> MGSSHHHHHSSGLVPRGSHMTTSAAS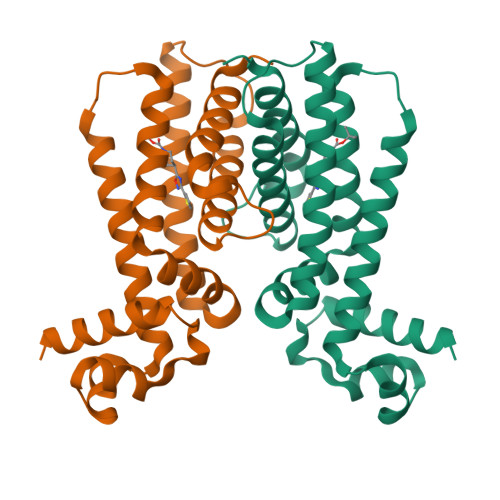QASLPRGRRTARPSGDDRELAILATAENLLEDRPLADISVDDLAKGAGISRPTFYFYFPSKEAVLLTLLDRVVNQADMALQTLAENPADTDRENMWRTGINVFFETFGSHKAVTRAGQAARATSVEVAELWSTFMQKWIAYTAAVIDAERDRGAAPRTLPAHELATALNLMNERTLFASFAGEQPSVPEARVLDTLVHIWVTSIYGENRMGSSHHHHHSSGLVPRGSHM>SNAMEPCLHPTLVDETSLVLYLDLARETGYRYVDVPFHW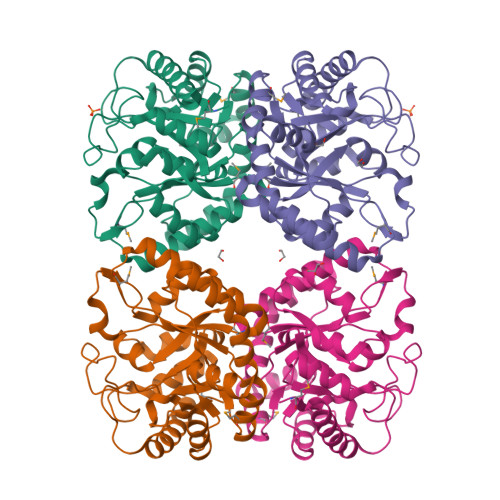LEAEAERHGDAAVEAMFQRRGLVLANLGLPLNLYDSEPVFLRELSLLPDRARLCARLGARSVTAFLWPSMDEEPVRYISQLARRIRQVAVELLPLGMRVGLEYVGPHHLRHRRYPFVQSLADLKTFWEAIGAPNVGALVDSYHWYTAGEHEDDLAQLPPEKVVYVHINDTRDAPEDAHDGKRLLPGDGRIPLVPFLRGLYLAGYRGPVAAEVLHETPLDGTGESRARLVRERLEKLIALAKG[2x]> ADKELKFLVVDDFSTMRRIVRNLLKELGFNNVEEAEDGVDALNKLQAGGYGFVISDWNMPNMDGLELLKTIRADGAMSALPVLMVTAEAKKENIIAAAQAGASGYVVKPFTAATLEEKLNKIFEKLGM;> TTEENSKSEAL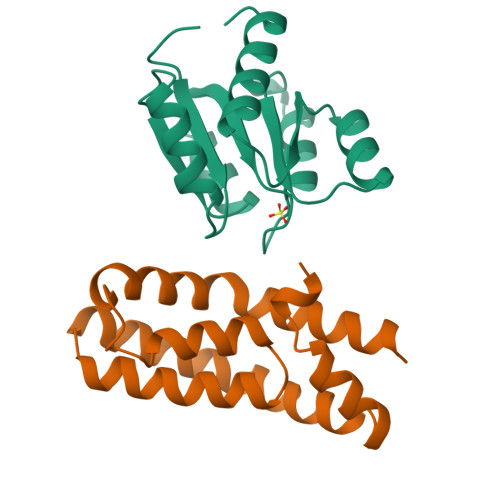LDIPMLEQYLELVGPKLITDGLAVFEKMMPGYVSVLESNLTAQDKKGIVEEGHKIKGAAGSVGLRHLQQLGQQIQSPDLPAWEDNVGEWIEEMKEEWRHDVEVLKAWVAKATKK>WLPHQRKVFDFYASQGVQYFTAFLIVSNFIFNCAEKEWDPYTDQLYQGLWRWGEFAFNTMFLIELLINFYGIAFCFWRYNWAWNTFDLVVVAIGTLTMAEAIGGNFMPPSMALIRNLRAFRIFRLFKRIKSLNKIIVSLGKAIPGVANAFVIMVIIMCIYAILGVEFYHMTGSDGTYVTYNDNVKRGLCTGDEVELGQCSLNQTVSSETARGYTYGEEYYGTFFRALYTLFQVLTGESWSEAVARPAVFESHYDSFGPVLFYVSFIIICQIVLINVVVAVLLDKMVEED[4x];> IAAIHNARRKKREAAAAHKA

Voltage-gated sodium (NaV) channels are responsible for the initiation and propagation of electrical signals in nerves, muscles, cardiomyocytes, and other excitable cells. Inactivation of the NaV channel terminates sodium influx and thus determines the availability of the channel. Interestingly, we have recently described an unexpected N-terminal helix (N-helix) mediated N-type fast inactivation of NaVEh from the coccolithophore Emiliania huxleyi, which is mechanistically distinct from the IFM-motif mediated fast inactivation but similar to the ball-and-chain inactivation of potassium channels. Prolonged depolarization or repetitive depolarizing pulses over a duration of tens of seconds cause slow inactivation of NaV channel, a phenomenon that is significantly different from the fast inactivation in the context of onset and recovery rate.

To assess the potential Ca2+-dependent activation, we measured NaVEhWT currents in the presence of Ca2+ or EGTA using the whole-cell patch clamp recording of HEK293 cells. The NaVEh-expressing cells consistently generated robust inward currents regardless of with Ca2+ or EGTA. To further assess the potential regulation of NaVEh by Ca2+ from a structural aspect, we determined the cryo-EM structures of NaVEh in the presence of 2 mM Ca2+ (NaVEhWT_Ca) and 2 mM EGTA (NaVEhWT_EGTA), respectively. The resulting two structures are essentially identical with a root mean square deviation (RMSD) of 0.37 Å, and only subtle conformational shifts between the side-chains in the extracellular loops (ECLs) of the structures can be observed. These results confirm that Ca2+ has negligible effects on the function and structure of NaVEh. Within the SF of NaVEhWT, four E305 residues are properly orientated to form a ‘high-field strength’ (HFS) site that attracts extracellular hydrated Na+. In the presence of the N-helix, the channel activates in response to depolarizing pulses, then the N-helix quickly blocks the open activation gate, resulting in the fast inactivation of NaVEh.> MLLDDQLKYWVLLPISIVMVLTGVLKQYIMTLITGSSANEAQPRVKLTEWQYLQWAQLLIGNGGNLSSDAFAAKKEFLVKDLTEERHLAKAKQQDGSQAGEVPNPFNDPSMSNAMMNMAKGNMASFIPQTIIMWWVNHFFAGFILMQLPFPLTAKFKEMLQTGIICQDLDVRWVSSISWYFISVLGLNPVYNLIGLNDQDMGIQAGIGGPQGPQGPPQSQVDKAMHAMANDLTIIQHE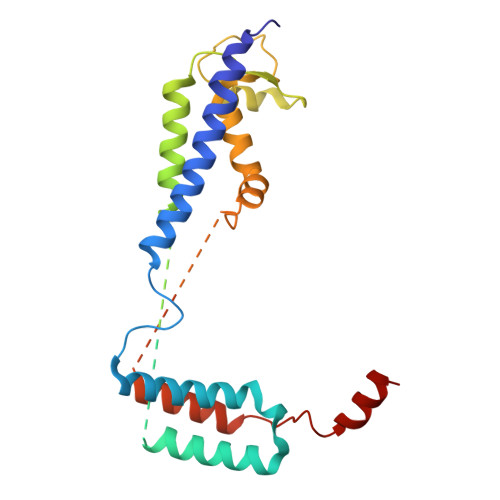TCLDNVEQRVLKQYM3-[2-[4-(4-fluorophenyl)carbonylpiperidin-1-yl]ethyl]-1~{H}-quinazoline-2,4-dione | C22 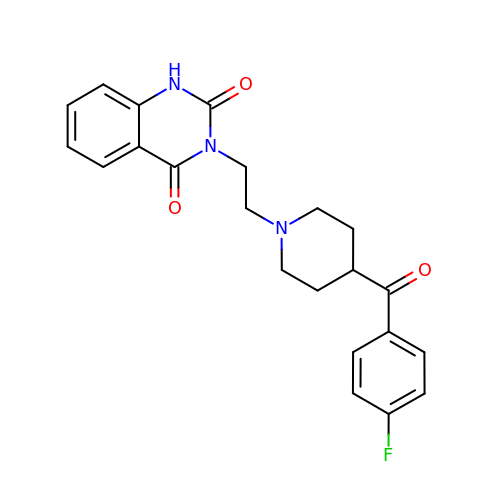H22 F N3 O3 | FPCCSQOGAWCVBH-UHFFFAOYSA-N> MKALILVGGFGTRLRPLTLSFPKPLVDFANKPMILHQIEALKAVGVDEVVLAINYQPEVMLNFLKDFETKLEIKIT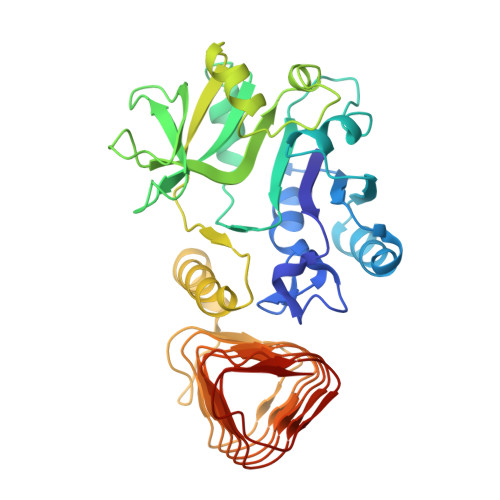CSQETEPLGTAGPLALARDKLLDGSGEPFFVLNSDVISEYPLKEMLEFHKSHGGEASIMVTKVDEPSKYGVVVMEESTGRVEKFVEKPKLYVGNKINAGIYLLNPSVLDKIELRPTSIEKETFPKIAAAQGLYAMVLPGFWMDIGQPRDYITGLRLYLDSLRKKSPAKLTSGPHIVGNVLVDETATIGEGCLIGPDVAIGPGCIVESGVRLSRCTVMRGVRIKKHACISSSIIGWHSTVGQWARIENMTILGEDVHVSDEIYSNGGVVLPHKEIKSNILKPEIVM>[4x]MKLSGVELRRVQMPLVAPFRTSFGTASVRELLLLRAVTPAGEGWGECVTIAGPLYSSEYNDGAEHVLRHYLIPALLAAEDITAAKVTPLLAKFKGHRMAKGALEMAVLDAELRAHERSFAAELGSVRDSVPCGVSV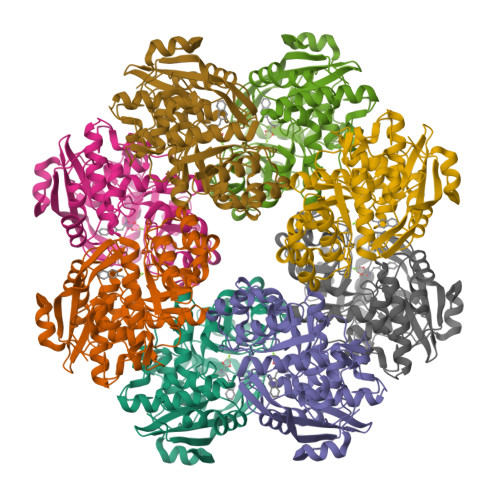GIMDTIPQLLDVVGGYLDEGYVRIKLKIEPGWDVEPVRAVRERFGDDVLLQVDANTAYTLGDAPQLARLDPFGLLLIEQPLEEEDVLGHAELARRIQTPICLDESIVSARAAADAIKLGAVQIVNIKPGRVGGYLEARRVHDVCAAHGIPVWCGDMIETGLGRAANVALASLPNFTLPGDTSASDRYYKTDITEPFVLSGGHLPVPTGPGLGVAPIPELLDEVTTAKVWIGS>MSGNMDEAVSGNMDEAVSAGKDVRIARWVATIAGLLGFVLSVSIPLLPVTQTTATLNWPQQGRLDNVTAPLISQAPLELTATVPCSVVRDLPPEGGLVFGTAPAEGRDAALNAMLVNVTETRVDVIVRNVVVASVNRDRVAGPDCQRIEITSNLDGTYADFVGLTQISGEDAGKLQRTGYPDPNLRPAIVGVFTDLTGPAPQGLSVSAEIDTRFTTHPTALKLAAMLLAIVSTVIALLALWRLDRLDGRRMHRLIPTRWRTVTAVDGVVVGGMAIWYVIGANSSDDGYILQMARTAEHAGYMANYFRWFGSPEDPFGWYYNVLALMTKVSDASIWIRLPDLICALICWLLLSREVLPRLGPAVAGSRAAMWAAGLVLLGAWMPFNNGLRPEGQIATGALITYVLIERAVTSGRLTPAALAITTAAFTLGIQPTGLIAVAALLAGGRPILRIVMRRRRLVGTWPLIAPLLAAGTVILAVVFADQTIATVLEATRIRTAIGPSQEWWTENLRYYYLILPTTDGAISRRVAFVFTAMCLFPSLFMMLRRKHIAGVARGPAWRLMGIIFATMFFLMFTPTKWIHHFGLFAAVGGAMAALATVLVSPTVLRSARNRMAFLSLVLFVLAFCFASTNGWWYVSNFGAPFNNSVPKVGGVQISAIFFALSAIAALWAFWLHLTRRTESRVVDRLTAAPIPVAAGFMVVVMMASMAIGVVRQYPTYSNGWANIRAFAGGCGLADDVLVEPDSNAGFLTPLPGAYGPLGPLGGEDPQGFSPDGVPDRIIAEAIRLNNPQPGTDYDWNRPIKLDEPGINGSTVPLPYGLDPKRVPVAGTYSTEAQQESRLSSAWYELPARDETERAAHPLVVITAAGTITGESVANGLTTGQTVDLEYATRGPDGTLVPAGRVTPYDVGPTPSWRNLRYPRSEIPDDAVAVRVVAEDLSLSQGDWIAVTPPRVPELQSVQEYVGSDQPVLMDWAVGLAFPCQQPMLHANGVTEVPKFRISPDYYAKLQSTDTWQDGINGGLLGITDLLLRASVMSTYLSQDWGQDWGSLRKFDTVVEATPAELDFGSQTHSGLYSPGPLRIRP[2x];>MAATQEEIIAGLAEIIEEVTGIEPSEVTPEKSFVDDLDIDSLSMVEIAVQTEDKYGVKIPDEDLAGLRTVGDVVAYIQKLEEENPEAAAALREKFAADQ[2x]

Furthermore, EmbB has been shown to play a key role in forming the characteristic terminal hexarabinofuranosyl motif of AG, which is the template for mycolylation. Together with the other Emb proteins (EmbA and EmbC), EmbB belongs to the glycosyltransferase C (GT-C) superfamily, whose structures comprises an N-terminal transmembrane domain and a C-terminal soluble domain located on the periplasmic side of the membrane. EmbB is observed as a dimer along with an acyl-carrier-protein (AcpM) associated with each protomer, thus forming a heterotetrameric EmbB2-AcpM2 complex. The EmbB protomers in the two states share common structural features which include two periplasmic domains (PDs) and 15 transmembrane helices (TMH) arranged into an approximately crescent-shaped bundle.

In this study, we have determined the structures of a substrate unbound EmbB2-AcpM2 complex in a presumed resting state and a donor DPA-bound pre-catalytic conformation which we define as the “active” state. Most significantly, the two EmbB protomers in the DPA bound complex are asymmetrically associated. Relative to the DPA-bound protomer, the other EmbB protomer is translated by ~16 Å along the dimer interface, and in the plane of the membrane. This change in subunit organization dramatically alters the dimer interface, in which, for instance, the distance between the pair of TMH11 at the interface has halved, resulting in a more compact active site. The whole of the DPA fits into this part of the map with the arabinose moiety and phosphate group fitting into a charged cavity just above the membrane surface. This cavity is bordered by PL2 which contains the catalytically relevant D(285)D(286)x motif; PL5 which is organized as two short α-helices (α5 and α6) and a following loop region; and the mixed α/β subdomain of PDC. For instance, the phosphate group is coordinated in place by R495PL5, while the arabinose moiety forms hydrogen bonds with E313PL2 and Q431PL4 which themselves are further stabilized by N304PL2 and Y320PL2. The last seven prenyl groups of DPA extend to the other half of the hydrophobic groove via extensive hydrophobic interactions with I421TMH7, V438TMH8, I448TMH8, I468TMH9 and I469TMH9 in the membrane space, with the end of the tail interacting with F670TM14 from the other EmbB protomer. Another structural rearrangement upon DPA binding, by comparing the structures of the two states, involves α6 in PL5, a short α helix that interacts with DPA, whereas in the resting state, this region is disordered. The DPA bound EmbB2-AcpM2 structure in this study represents an intermediate state before C1 of DPA reaches the optimal position for catalysis.>[9x]GSGSVIPPENFSHVVGEIYRSSFPRQENFSFLHERLKLKSILVLIPEEYPQENLNFLKLTGIKLYQ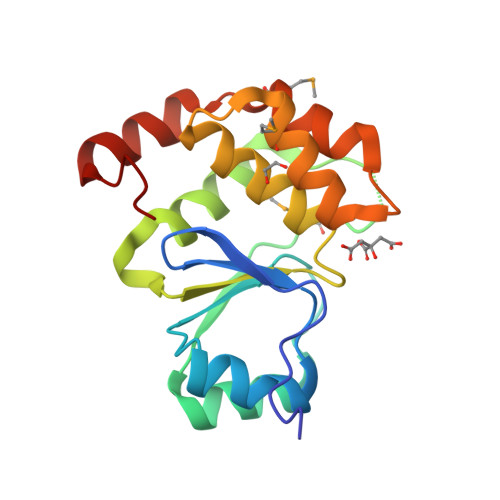VGMSGNKEPFVNIPSHLLTKALEIVLNPANQPILIHCNRGKHRTGCLIGCIRKLQNWSLTMIFDEYRRFAFPKARALDQQFIEMYDDDEIKRIASKNNWLPLQW>[2x]MSLVRSKAPLRLGLAGGGSDVSPYSDIYGGLILNATINLYAYCTIEETNSGRIEINAYDAQCCKSYLSMSQLEIDGEASLIKGVYNRIIRDYRLEPKSFKITTYNDAPAGSGLGTSSTMVVCILKAFIEWLSLPLGDYETSRLAYEIERKDLGLSGGKQDQYAAAFGGFNYMEFLQNDLVIVNPLKMKRWIVDELESSMVLYFTGRSRSSAAIINEQKKNTSEGNQTAIEAMHKIKQ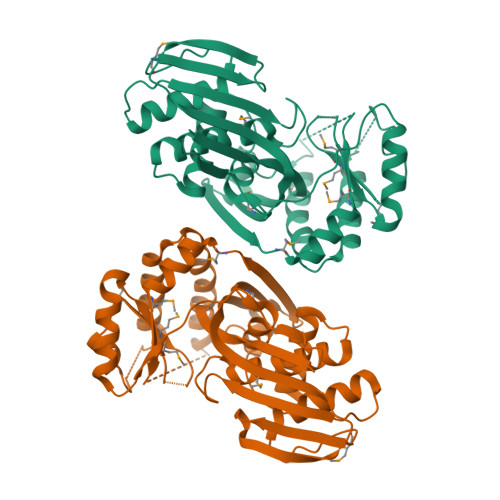SAIDTKLALLKGDVGEFARILGEGWENKKKMAGAITNPMIQEAFDVATGAGAMAGKVSGAGGGGFIMFVVEPTRKEEVVRALNNLNGFVMPFQFIDDGAHGWKIYSTDKVQKEGHHHHHH>[3x]MVNQLIEPYGGTLVNLIDPEKREALKHEALSLPSLDLDWQQQCELEMLMTGAYSPLTGFMTRAQCARVESAQQLDDGSFWPSPITLTSRDRALADRRPGERLALRDGEGYMLAILTLSDVWKDGERWHLAGEVEGAALPPHPDFVSLRATPAELRALFVRRGWRRIIAWQARQPMHRAQYEFCLKSAIENEANLLLHPQVGGDITEAPAYFGLVRSFLAIRDRFPAATTQLSLLPAPPPEASGRALLLRAIVARNFGCSLLIAGGEHQPDGGDCRRGEDLTQNRVDPSVAERAEKIGVRLIAYPRMVYVEDRAEHLPEAEAPQGARLLTLSGEEFQRRMRAGLKIPEWYSFPEVLAELHRQTPPRERQGFTVFFTGLSGAGKSTLARALAARLMEMGGRCVT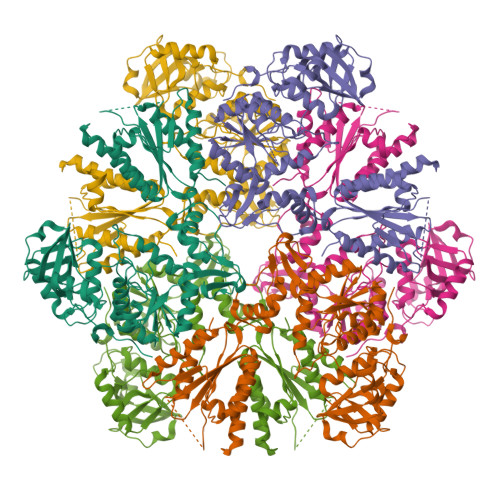LLDGDIVRRHLSSELGFSKAHRDVNVRRIGFVASEITKNRGIAICAPIAPYRQTRRDVRAMIEAVGGFVEIHVATPIETCESRDRKGLYAKARAGLIPEFTGVSDPYEVPETPELAIDTTGLAIDEAVQQILLKLEHEGYLRLEHHHHHH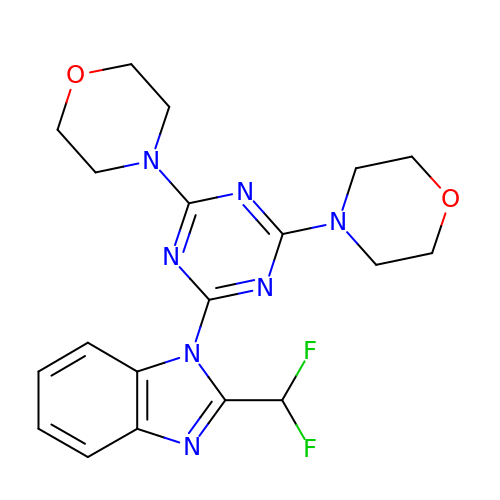2-(difluoromethyl)-1-(4,6-dimorpholin-4-yl-1,3,5-triazin-2-yl)-1H-benzimidazole | C19 H21 F2 N7 O2 | HGVNLRPZOWWDKD-UHFFFAOYSA-N>[3x]MKIEEVKSTTKTQRIASHSHVKGLGLDESGLAKQAASGLVGQENAREACGVIVELIKSKKMAGRAVLLAGPPGTGKTALALAIAQELGSKVPFCPMVGSEVYSTEIKKTEVLMENFRRAIGLRIKETKEVYEGEVTELTPCETENPMGGYGKTISHVIIGLKTAKGTKQLKLDPSIFESLQKERVEAGDVIYIEANSGAVKRQGRCDTYATEFDLEAEEYVPLPKGDVHKKKEIIQDVTLHDLDVANARPQGGQDILSMMGQLMKPKKTEITDKLRGEINKVVNKYIDQGIAELVPGVLFVDEVHMLDIECFTYLHRALESSIAPIVIFASNRGNCVIRGTEDITSPHGIPLDLLDRVMIIRTMLYTPQEMKQIIKIRAQTEGINISEEALNHLGEIGTKTTLRYSVQLLTPANLLAKINGKDSIEKEHVEEISELFYDAKSSAKILADQQDKYMK;>[3x]MATVTATTKVPEIRDVTRIERIGAHSHIRGLGLDDALEPRQASQGMVGQLAARRAAGVVLEMIREGKIAGRAVLIAGQPGTGKTAIAMGMAQALGPDTPFTAIAGSEIFSLEMSKTEALTQAFRRSIGVRIKEETEIIEGEVVEIQIDRPATGTGSKVGKLTLKTTEMETIYDLGTKMIESLTKDKVQAGDVITIDKATGKISKLGRSFTRARDYDAMGSQTKFVQCPDGELQKRKEVVHTVSLHEIDVINSRTQGFLALFSGDTGEIKSEVREQINAKVAEWREEGKAEIIPGVLFIDEVHMLDIESFSFLNRALESDMAPVLIMATNRGITRIRGTSYQSPHGIPIDLLDRLLIVSTTPYSEKDTKQILRIRCEEEDVEMSEDAYTVLTRIGLETSLRYAIQLITAASLVCRKRKGTEVQVDDIKRVYSLFLDESRSTQYMKEYQDAFLFNELKGETMDTS;> MTTLVLDNGAYNAKIGYSHENVSVIPNCQFRSKTARLKTFTANQIDEIKDPSGLFYILPFQKGYLVNWDVQRQVWDYLFGKEMYQVDFLDTNIIITEPYFNFTSIQESMNEILFEEYQFQAVLRVNAGALSAHRYFRDNPSELCCIIVDSGYSFTHIVPYCRSKKKKEAIIRINVGGKLLTNHLKEIISYRQLHVMDETHVINQVKEDVCYVSQDFYRDMDIAKLKGEENTVMIDYVLPDFSTIKKGFCKPREEMVLSGKYKSGEQILRLANERFAVPEILFNPSDIGIQEMGIPEAIVYSIQNLPEEMQPHFFKNIVLTGGNSLFPGFRDRVYSEVRCLTPTDYDVSVVLPENPITYAWEGGKLISENDDFEDMVVTREDYEENGHSVCEEKFDI;> MQSSPSPAHPQLPVLQTQMVSDGMTGSNPVSPASSSSPASSGAGGISPQHIAQDSSLDGPPGPPDGATVPLEGFSLSQAADLANKGPKWEKSHAEIAEQAKHEAEIETRIAELRKEGFWSLKRLPKVPEPPRPKGHWDYLCEEMQWLSADFAQERRWKRGVARKVVRMVIRHHEEQRQKEERARREEQAKLRRIASTMAKDVRQFWSNVEKVVQFKQQSRLEEKRKKALDLHLDFIVGQTEKYSDLLSQSLNQPLTSSKAGSSPCLGSSSAASSPPPPASRLDDEDGDFQPQEDEEE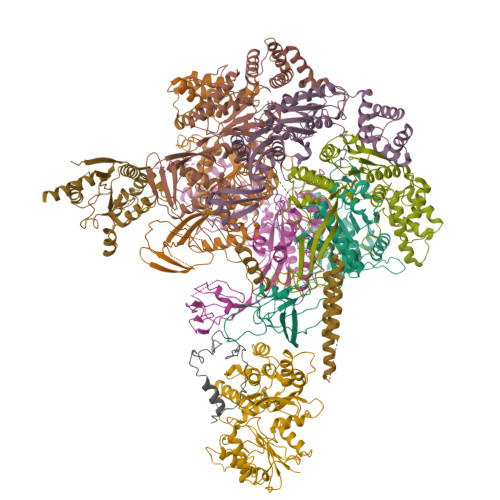DDEETIEVEEQQEGNDAEAQRREIELLRREGELPLEELLRSLPPQLLEGPSSPSQTPSSHDSDTRDGPEEGAEEEPPQVLEIKPPPSAVTQRNKQPWHPDEDDEEFTANEEEAEDEEDTIAAEEQLEGEVDHAMELSELAREGELSMEELLQQYAGAYAPGSGSSEDEDEDEVDANSSDCEPEGPVEAEEPPQEDSSSQSDSVEDRSEDEEDEHSEEEETSGSSASEESESEESEDAQSQSQADEEEEDDDFGVEYLLARDEEQSEADAGSGPPTPGPTTLGPKKEITDIAAAAESLQPKGYTLATTQVKTPIPLLLRGQLREYQHIGLDWLVTMYEKKLNGILADEMGLGKTIQTISLLAHLACEKGNWGPHLIIVPTSVMLNWEMELKRWCPSFKILTYYGAQKERKLKRQGWTKPNAFHVCITSYKLVLQDHQAFRRKNWRYLILDEAQNIKNFKSQRWQSLLNFNSQRRLLLTGTPLQNSLMELWSLMHFLMPHVFQSHREFKEWFSNPLTGMIEGSQEYNEGLVKRLHKVLRPFLLRRVKVDVEKQMPKKYEHVIRCRLSKRQRCLYDDFMAQTTTKETLATGHFMSVINILMQLRKVCNHPNLFDPRPVTSPFITPGICFSTASLVLRATDVHPLQRIDMGRFDLIGLEGRVSRYEADTFLPRHRLSRRVLLEVATAPDPPPRPKPVKMKVNRMLQPVPKQEGRTVVVVNNPRAPLGPVPVRPPPGPELSAQPTPGPVPQVLPASLMVSASPAGPPLIPASRPPGPVLLPPLQPNSGSLPQVLPSPLGVLSGTSRPPTPTLSLKPTPPAPVRLSPAPPPGSSSLLKPLTVPPGYTFPPAAATTTSTTTATATTTAVPAPTPAPQRLILSPDMQARLPSGEVVSIGQLASLAQRPVANAGGSKPLTFQIQGNKLTLTGAQVRQLAVGQPRPLQRNVVHLVSAGGQHHLISQPAHVALIQAVAPTPGPTPVSVLPSSTPSTTPAPTGLSLPLAANQVPPTMVNNTGVVKIVVRQAPRDGLTPVPPLAPAPRPPSSGLPAVLNPRPTLTPGRLPTPTLGTARAPMPTPTLVRPLLKLVHSPSPEVSASAPGAAPLTISSPLHVPSSLPGPASSPMPIPNSSPLASPVSSTVSVPLSSSLPISVPTTLPAPASAPLTIPISAPLTVSASGPALLTSVTPPLAPVVPAAPGPPSLAPSGASPSASALTLGLATAPSLSSSQTPGHPLLLAPTSSHVPGLNSTVAPACSPVLVPASALASPFPSAPNPAPAQASLLAPASSASQALATPLAPMAAPQTAILAPSPAPPLAPLPVLAPSPGAAPVLASSQTPVPVMAPSSTPGTSLASASPVPAPTPVLAPSSTQTMLPAPVPSPLPSPASTQTLALAPALAPTLGGSSPSQTLSLGTGNPQGPFPTQTLSLTPASSLVPTPAQTLSLAPGPPLGPTQTLSLAPAPPLAPASPVGPAPAHTLTLAPASSSASLLAPASVQTLTLSPAPVPTLGPAAAQTLALAPASTQSPASQASSLVVSASGAAPLPVTMVSRLPVSKDEPDTLTLRSGPPSPPSTATSFGGPRPRRQPPPPPRSPFYLDSLEEKRKRQRSERLERIFQLSEAHGALAPVYGTEVLDFCTLPQPVASPIGPRSPGPSHPTFWTYTEAAHRAVLFPQQRLDQLSEIIERFIFVMPPVEAPPPSLHACHPPPWLAPRQAAFQEQLASELWPRARPLHRIVCNMRTQFPDLRLIQYDCGKLQTLAVLLRQLKAEGHRVLIFTQMTRMLDVLEQFLTYHGHLYLRLDGSTRVEQRQALMERFNADKRIFCFILSTRSGGVGVNLTGADTVVFYDSDWNPTMDAQAQDRCHRIGQTRDVHIYRLISERTVEENILKKANQKRMLGDMAIEGGNFTTAYFKQQTIRELFDMPLEEPSSSSVPSAPEEEEETVASKQTHILEQALCRAEDEEDIRAATQAKAEQVAELAEFNENDGFPAGEGEEAGRPGAEDEEMSRAEQEIAALVEQLTPIERYAMKFLEASLEEVSREELKQAEEQVEAARKDLDQAKEEVFRLPQEEEEGPGAGDESSCGTGGGTHRRSKKAKAPERPGTRVSERLRGARAETQGANHTPVISAHQTRSTTTPPRCSPARERVPRPAPRPRPTPASAPAAIPALVPVPVSAPVPISAPNPITILPVHILPSPPPPSQIPPCSSPACTPPPACTPPPAHTPPPAQTCLVTPSSPLLLGPPSVPISASVTNLPLGLRPEAELCAQALASPESLELASVASSETSSLSLVPPKDLLPVAVEILPVSEKNLSLTPSAPSLTLEAGSIPNGQEQEAPDSAEGTTLTVLPEGEELPLCVSESNGLELPPSAASDEPLQEPLEADRTSEELTEAKTPTSSPEKPQELVTAEVAAPSTSSSATSSPEGPSPARPPRRRTSADVEIRGQGTGRPGQPPGPKVLRKLPGRLVTVVEEKELVRRRRQQRGAASTLVPGVSETSASPGSPSVRSMSGPESSPPIGGPCEAAPSSSLPTPPQQPFIARRHIELGVTGGGSPENGDGALLAITPPAVKRRRGRPPKKNRSPADAGRGVDEAPSSTLKGKTNGADPVPGPETLIVADPVLEPQLIPGPQPLGPQPVHRPNPLLSPVEKRRRGRPPKARDLPIPGTISSAGDGNSESRTQPPPHPSPLTPLPPLLVCPTATVANTVTTVTISTSPPKRKRGRPPKNPPSPRPSQLPVLDRDSTSVLESCGLGRRRQPQGQGESEGSSSDEDGSRPLTRLARLRLEAEGMRGRKSGGSMVVAVIQDDLDLADSGPGGLELTPPVVSLTPKLRSTRLRPGSLVPPLETEKLPRKRAGAPVGGSPGLAKRGRLQPPSPLGPEGSVEESEAEASGEEEEGDGTPRRRPGPRRLVGTTNQGDQRILRSSAPPSLAGPAVSHRGRKAKT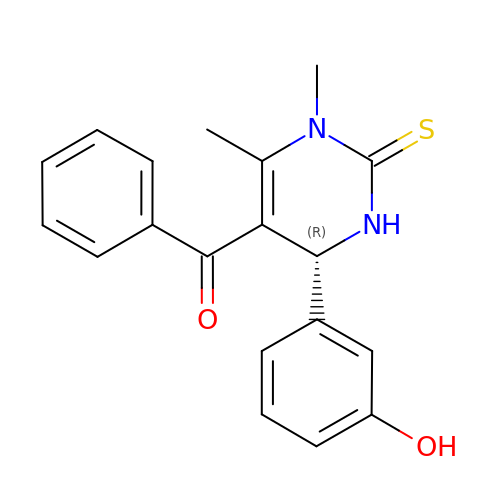[(4R)-4-(3-HYDROXYPHENYL)-1,6-DIMETHYL-2-THIOXO-1,2,3,4-TETRAHYDROPYRIMIDIN-5-YL](PHENYL)METHANONE | C19 H18 N2 O2 S | JGBBILLMZPWNFU-QGZVFWFLSA-N>TDTTPPTITLPQEVIAYRGEEFEFFVETTDDSGRVNRVIVRNIEGADNSTYLDPNWIRYSTDNLSVPGNATPANPLRTRVYGIVPINHGVGPGDRYTKYVRAEDAAGNITALVDKQSERFVLVIRPQTEKYTPQVPTLTYVQNANSLTQTDKDAVIAAVKSANPNLPATSTYSVSENGTVTITYPDGSTDTIAAAQTVDTDRVAPVFVDEGRDYIFYRGEEGTAELHFYDNSGKITNVNFAGDLAASSTYNTLLGLGFTFNTPNINNPNNATEQNPLVTTIRGTIPKSLPAGPGGKYTFKVRATDASGLTSEAKIFRIVFANQTDKYTPNNPGSLTGVLNPQQLSTSEKTAIEEKVRAANTGNLPNNVQYVVNNDGSVTVIYPDDTPASRSRDTITADRTVQDLRPRNS[2x]

The serine-rich repeat (SRR) adhesins are a family of bacterial cell-surface glycoproteins containing two sequence motifs where serine constitutes ∼50% of the sequence. The binding region from S. sanguinis strain SK1 (residues 252–660 and termed SK1BR) differs from structurally characterized Siglec-containing binding regions in two ways. First, it contains two copies of the Siglec and Unique domains in tandem (SK1Siglec1-SK1Unique1-SK1Siglec2-SK1Unique2) with sequence identity/similarity of 39%/56% between the two Siglec domains and 44%/50% between the two Unique domains. The second way that SK1BR differs from other structurally characterized Siglec-like binding regions is that each of the putative Siglec domains of SK1BR contains a noncanonical YTRY sialic acid–binding sequence motif that lacks the central Thr-Arg deemed to be critical for binding in other Siglec-like adhesins.

To develop hypotheses for how SK1BR binds to sialoglycans, we began by determining its X-ray crystal structure using molecular replacement methods. The tandem repeats of unliganded SK1BR fold independently, and slight angles between the domains yield an elongated and overall arc shape. The limits of the domains can be clearly distinguished as SK1Siglec1 (residues 252–377), SK1Unique1 (residues 378–453), SK1Siglec2 (residues 454–573), and SK1Unique2 (residues 574–660). As is anticipated from the amino acid sequence conservation, the individual Siglec domains and Unique domains exhibit structural similarity, with RMS deviations in Cα position of 1.058 Å between SK1Siglec1 and SK1Siglec2 and 0.639 Å between SK1Unique1 and SK1Unique2. We identified disproportionately large structural deviations in the CD, EF, and FG selectivity loops that surround the putative sialoglycan-binding pockets, which contain different numbers of residues, with the FG loop of SK1Siglec2 being so short that it is effectively absent. In the CD loop, this also manifests as a difference in secondary structure in which the CD loop of SK1Siglec1 lacks secondary structure, whereas the CD loop of SK1Siglec2 folds into an α-helix. In addition, the CD loop of SK1Siglec2 is displaced from the binding pocket when compared with the CD loop of SK1Siglec1. Together, these differences in loop length and structure result in a larger and more open binding site as compared with SK1Siglec1. In the unliganded state, we observe that the selectivity loops have elevated temperature factor values as compared with the V-set Ig fold that forms the core of the Siglec domain, suggesting that they have increased mobility.>[8x]MANAERMITRVHSQRERLNETLVSERNEVLALLSRVEAKGKGILQQNQIIAEFEALPEQTRKKLEGGPFFDLLKSTQEAIVLPPWVALAVRPRPGVWEYLRVNLHALVVEELQPAEFLHFKEELVDGVKNGNFTLELDFEPFNASIPRPTLHKYIGNGVDFLNRHLSAKLFHDKESLLPLLKFLRLHSHQGKNLMLSEKIQNLNTLQHTLRKAEEYLAELKSETLYEEFEAKFEEIGLERGWGDNAERVLDMIRLLLDLLEAPDPCTLETF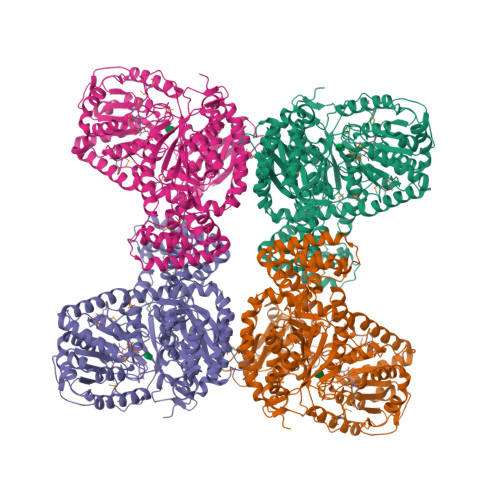LGRVPMVFNVVILSPHGYFAQDNVLGYPDTGGQVVYILDQVRALEIEMLQRIKQQGLNIKPRILILTRLLPDAVGTTCGERLERVYDSEYCDILRVPFRTEKGIVRKWISRFEVWPYLETYTEDAAVELSKELNGKPDLIIGNYSDGNLVASLLAHKLGVTQCTIAHALEKTKYPDSDIYWKKLDDKYHFSCQFTADIFAMNHTDFIITSTFQEIAGSKETVGQYESHTAFTLPGLYRVVHGIDVFDPKFNIVSPGADMSIYFPYTEEKRRLTKFHSEIEELLYSDVENKEHLCVLKDKKKPILFTMARLDRVKNLSGLVEWYGKNTRLRELANLVVVGGDRRKESKDNEEKAEMKKMYDLIEEYKLNGQFRWISSQMDRVRNGELYRYICDTKGAFVQPALYEAFGLTVVEAMTCGLPTFATCKGGPAEIIVHGKSGFHIDPYHGDQAADTLADFFTKCKEDPSHWDEISKGGLQRIEEKYTWQIYSQRLLTLTGVYGFWKHVSNLDRLEARRYLEMFYALKYRPLAQAVPLAQDDVEHHHHHH>GSMGLYFSSLDSSIDILQKRAQELIENINKSRQKDHALMTNFRNSLKTKVSDLTEKLEERIYQIYNDHNKIIQEKLQEFTQKMAKISHLETELKQVCHSVETVYKDLCLQPE[2x];>GSMGKDEALEKDLNDVSKEINLMLSTYAKLLSERAAVDASYIDEIDELFKEANAIENFLIQKREFLRQR[2x]

The synaptonemal complex (SC) is a supramolecular protein assembly that mediates synapsis between homologous chromosomes during meiosis. SC elongation along the chromosome length (up to 24 μm) depends on its midline α-fibrous component SYCE2-TEX12. SYCE2-TEX12’s building-blocks are 2:2 coiled-coils which dimerise into 4:4 hetero-oligomers and interact end-to-end and laterally to form 10-nm fibres, which intertwine within 40-nm bundled micrometre-long fibres that define the SC’s midline structure. Thus, SYCE2-TEX12 exhibits behaviour typical of cytoskeletal proteins to provide an α-fibrous SC backbone that structurally underpins synaptic elongation along meiotic chromosomes.

We obtained an alternative crystal form of SYCE2-TEX12 ΔCtip core, which diffracted anisotropically to 3.33–6.00 Å resolution, and was solved by molecular replacement using a three-helical bundle of the 2:2 structure as a search model. This revealed a 4:4 structure in which two 2:2 complexes interact laterally, through tessellation of S-shaped SYCE2 dimers, to create a molecule of the same length (14 nm) but twice as wide (4 nm) as individual 2:2 complexes. The 2:2 crystal structure is largely retained by the two interacting 2:2 complexes (r.m.s. deviation = 1.91), which seamlessly generate an SYCE2 tetrameric core with staggered TEX12 chains arranged on opposing surfaces. In common with the 2:2 structure, S2C sequences were missing from electron density, meaning that pairs of truncated SYCE2 and TEX12 C-termini are juxtaposed at both ends of the 4:4 molecule. The observed tessellation of 2:2 complexes provides an enticing mechanism for assembly of a 4:4 complex from structurally intact obligate 2:2 molecules, in agreement with our biochemical findings. The 4:4 crystal structure lacks TEX12’s C-terminal tip, which is required for 4:4 assembly in solution, suggesting that this conformation was supported by the crystal lattice. We reasoned that the tessellating interface likely drives 4:4 assembly of the wild-type protein and is stabilised in solution by additional TEX12 Ctip interactions. The crystal lattice of the 4:4 structure is a fibrous array in which 4:4 molecules are arranged in end-to-end chains, with 1-nm gaps between juxtaposed C-termini, and a lateral stagger. Thus, the lateral tessellating interaction of 2:2 complexes within the 4:4 crystal structure describes the underlying architecture of the wild-type 4:4 assembly.>QSVCAGTENKLSSLSDLEQQYRALRKYYENCEVVMGNLEITSIEHNRDLSFLRSVREVTGYVLVALNQFRYLPLENLRIIRGTKLYEDRYALAIFLNYRKDGNFGLQELGLKNLTEILNGGVYVDQNKFLCYADTIHWQDIVRNPWPSNLTLVSTNGSSGCGRCHKSCTGRCWGPTENHCQTLTRTVCAEQCDGRCYGPYVSDCCHRECAGGCSGPKDTDCFACMNFNDSGACVTQCPQTFVYNPTTFQLEHN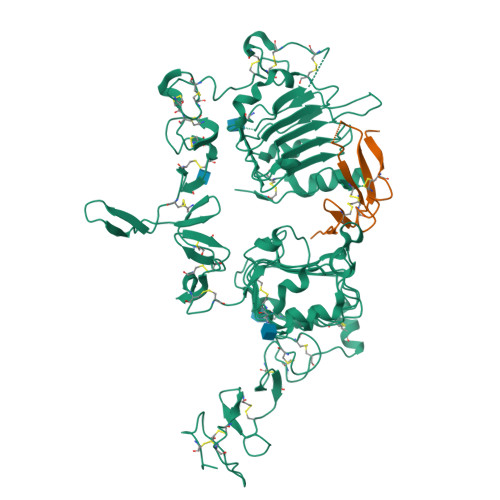FNAKYTYGAFCVKKCPHNFVVDSSSCVRACPSSKMEVEENGIKMCKPCTDICPKACDGIGTGSLMSAQTVDSSNIDKFINCTKINGNLIFLVTGIHGDPYNAIEAIDPEKLNVFRTVREITGFLNIQSWPPNMTDFSVFSNLVTIGGRVLYSGLSLLILKQQGITSLQFQSLKEISAGNIYITDNSNLCYYHTINWTTLFSTINQRIVIRDNRKAENCTAEGMVCNHLCSSDGCWGPGPDQCLSCRRFSRGRICIESCNLYDGEFREFENDSICVECDPQCEKMEDGLLTCHGPGPDNCTKCSHFKDGPNCVEKCPDGLQGANSFIFKYADPDRECHPCHPNCTQGCNGPTSHDCIYYPWTG[6x];>GTSHLVKCAEKEKTFCVNGGECFMVKDLSNPSRYLCKCPNEFTGDRCQNYVMASF[6x]3-PHENYLPROPANAL 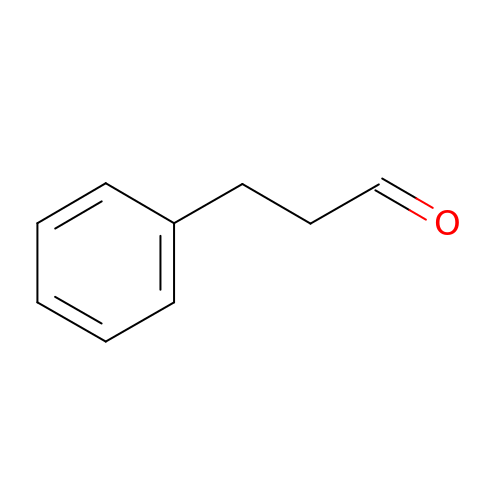| C9 H10 O | YGCZTXZTJXYWCO-UHFFFAOYSA-N> GELFRGVLHISSNILDCANDNWWCSMLDLDTSDWEPLTHSNRLMAIYLSNVASRLDFTGGPLAGCLYFFQVECNKFEEGYHIHVVIGGPGLNARNLTVCVEGLFNNVLYHLVNESVKLKFLPGMTTKGKYFRDGEQFIENYLMKKIPLNVVWCVTNIDGYIDTCISASF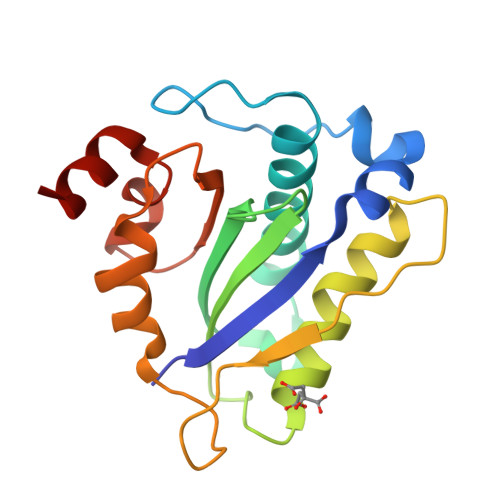RRGACHA The 8-carbon sugar 3-deoxy-d-manno-oct-2-ulosonic acid (Kdo) is a conserved structural element of the lipopolysaccharide (LPS) of Gram-negative bacteria. Prior to its linkage to the lipid A moiety by the Kdo transferase (WaaA), CMP-Kdo synthetase (CKS, EC 2.7.7.38) activates Kdo using CTP in a Mg2+-dependent reaction that results in the formation of CMP-Kdo and pyrophosphate. Crystal structures of LCKS and KCKS from E. coli as well as of LCKS from Haemophilus influenze (HI-LCKS) have been reported, displaying either no or one magnesium ion in the active site. These structures show that CTP binds to a nucleotide-binding fold located in the N-terminal domain of the enzyme, whereas parts of the C-terminal domain are involved in Kdo binding and the formation of the homodimer interface. In the present study, we describe the enzymatic properties, the crystallization, and the X-ray crystal structure of LCKS from the hyperthermophilic organism Aquifex aeolicus (AA-LCKS) in complex with CTP at 2.10 Å resolution and show for the first time that two Mg2+ ions are present in the active site of the enzyme.

The asymmetric unit (AU) of the AA-LCKS-CTP crystal structure contains three molecules arranged into one-and-a-half homodimers. Each polypeptide chain folds into a U-shaped molecule with a central, predominantly parallel, β-sheet surrounded by α-helices. The two arms of the U-shaped molecule are formed by the N- (residues 2–91 and 220–234) and C-terminal (residues 100–210) domain, respectively, the latter being responsible for homodimer formation and Kdo binding. Compared to the previously determined ternary EC-LCKS-CTP-2β-deoxy-Kdo crystal structure, AA-LCKS adopts a more open conformation with a larger groove between the two domains. R10, T14, R15, and K19 of the CTP loop bind to the nucleotide's triphosphate group, which adopts a staggered conformation and harbors a Mg2+ ion (Mg-B) with octahedral coordination geometry. In the AA-LCKS-CTP crystal structure, an additional Mg2+ ion (Mg-A) is present between the strictly conserved side chains of D219 and D95. The octahedral coordination geometry in this case is completed by interactions with the CTP α-phosphate group and surrounding water molecules. Furthermore, only Mg-A is connected to the protein via D95 and D219, while Mg-B interacts exclusively with the triphosphate moiety of the CTP and additional water molecules. The crystal structure of AA-LCKS provides the first direct structural evidence that two Mg2+ ions are recruited to the active site, strongly supporting the two-metal-ion scenario. Moreover, the structure demonstrates clearly that Mg-A binding does not depend on the presence of the regular Kdo substrate, as was suggested for EC-LCKS.

>[3x]MRRAVIIPARLGSTRLKEKPLKNLLGKPLIRWVVEGLVKTGERVILATDSERVKEVVEDLCEVFLTPSDLPSGSDRVLYVVRDLDVDLIINYQGDEPFVYEEDIKLIFRELEKGERVVTLARKDKEAYERPEDVKVVLDREGYALYFSRSPIPYFRKNDTFYPLKHVGIYGFRKETLMEFGAMPPSKLEQIEGLEQLRLLENGIKIKVLITENYYHGVDTEEDLKIVEEKLKNL[(3,7,11-TRIMETHYL-DODECA-2,6,10-TRIENYLOXYCARBAMOYL)-METHYL]-PHOSPHONIC 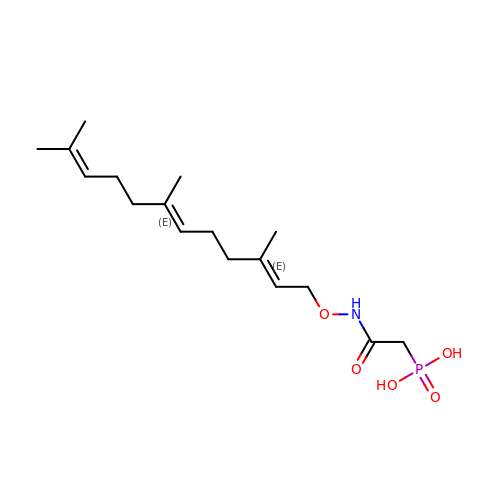ACID | C17 H30 N O5 P | JAOBYUCYSAOLHS-XGGJEREUSA-N>GSHGGS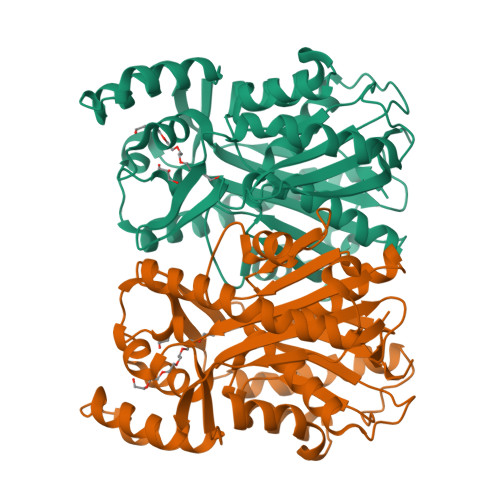GFMATLCRPSVSVPEHVITMEETLELARRRHTDHPQLPLALRLIENTGVRTRHIVQPIEDTLEHPGFEDRNKVYEREAKSRVPAVIQRALDDAELLATDIDVIIYVSCTGFMMPSLTAWLINEMGFDSTTRQIPIAQLGCAAGGAAINRAHDFCTAYPEANALIVACEFCSLCYQPTDLGVGSLLCNGLFGDGIAAAVVRGRGGTGVRLERNGSYLIPKTEDWIMYDVKATGFHFLLDKRVPATMEPLAPALKELAGEHGWDASDLDFYIVHAGGPRILDDLSTFLEVDPHAFRFSRATLTEYGNIASAVVLDALRRLFDEGGVEEGARGLLAGFGPGITAEMSLGCWQTADVRRGIRQDVTRTAARGVSRRVRQA[2x]> MAFAHFVLIHTICHGAWIWHKLKPLLEALGHKVTALDLAASGVDPRQIEEIGSF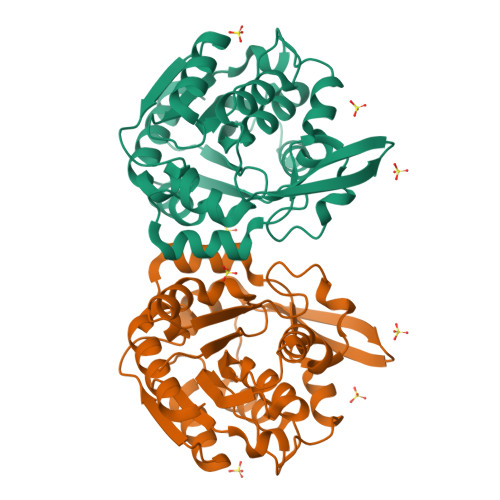DEYSEPLLTFLEALPPGEKVILVGESCGGLNIAIAADKYCEKIAAAVFHNSVLPDTEHCPSYVVDKLMEVFPDWKDTTYFTYTKDGKEITGLKLGFTLLRENLYTLCGPEEYELAKMLTRKGSLFQNILAKRPFFTKEGYGSIKKIYVWTDQDEIFLPEFQLWQIENYKPDKVYKVEGGDHLLQLTKTKEIAEILQEVADTYN>GTHMRKGVDLVTAGTPGENTTPEARVLVVDDEANIVELLSVSLKFQGFEVYTATNGAQALDRARETRPDAVILDVMMPGMDGFGVLRRLRADGIDAPALFLTARDSLQDKIAGLTLGGDDYVTKPFSLEEVVARLRVILRRAGKGNKEPRNVRLTFADIELDEETHEVWKAGQPVSLSPTEFTLLRYFVINAGTVLSKPKILDHVWRYDFGGDVNVVESYVSYLRRKIDTGEKRLLHTLRGVGYVLR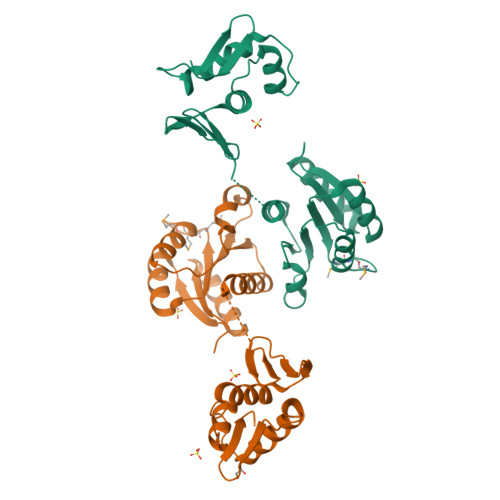EPR[2x]>GPGSMSLFKARDWWSTILGDKEEFDQGCLCLANVDNSGNGQDKIIVGSFMGYLRIFSPHPAKTGDGAQAEDLLLEVDLRDPVLQVEVGKFVSGTEMLHLAVLHSRKLCVYSVSGTLGNVEHGNQCQMKLMYEHNLQRTACNMTYGSFGGVKGRDLICIQSMDGMLMVFEQESYAFGRFLPGFLLPGPLAYSSRTDSFLTVSSCQQVESYKYQVLAFATDADKRQETEQQKLGSGKRLVVDWTLNIGEQALDICIVSFNQSASSVFVLGERNFFCLKDNGQIRFMKKLDWSPSCFLPYCSVSEGTINTLIGNHNNMLHIYQDVT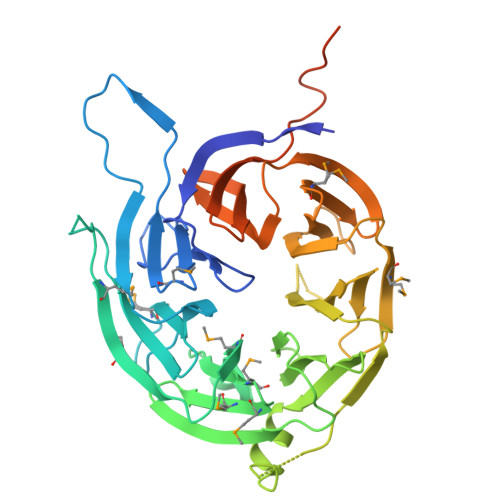LKWATQLPHIPVAVRVGCLHDLKGVIVTLSDDGHLQCSYLGTDPSLFQAPNVQSRELNYDELDVEMKELQKIIKDVNKSQGVWPMTER[2x]> MTTPSMEDYIEQIYMLIEEKGYARVSDIAEALAVHPSSVTKMVQKLDKDEYLIYEKYRGLVLTSKGKKIGKRLVYRHELLEQFLRIIGVDEEKIYNDVEGIEHHLSW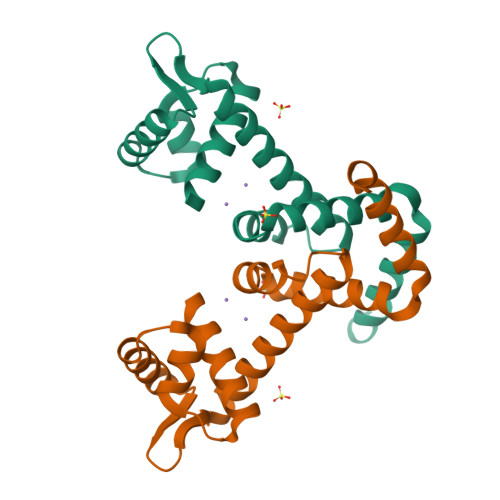NSIDRIGDLVQYFEEDDARKKDLKSIQKKTEHHNQ5'-(D-alanylamino)-5'-deoxyuridine 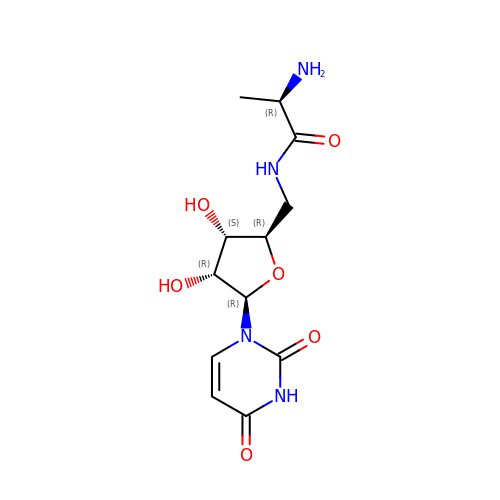| C12 H18 N4 O6 | DKBBANYKDGGYBY-LODYRLCVSA-N>[2x]GSHMNQTNLDDTLDVLNDLLQTSKDGEAGFHACAEDLRDPQLKAAMLEQSRDCAAAADELERIVLELGGKPKDSTSFAGDLHRRWVD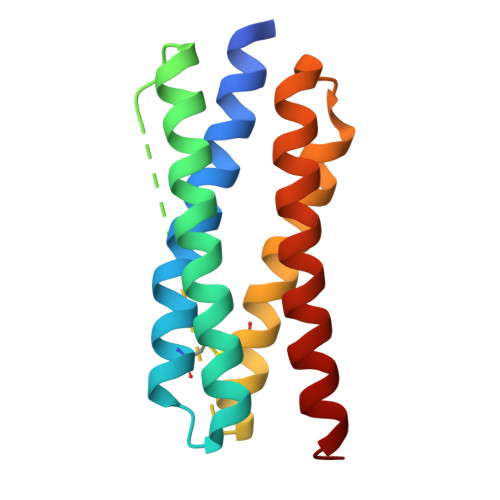LKSLVTGKDEEAVLNECERGEDVAKHRYQAALEKSLPAEIHQVIERQYQGVLRHHDRVRALRDARA>MGSSHHHHHHSQDPGFEFTLMVVGESGLGKSTLINSLFLTDLYSPEYPGPSHRIKKTVQVEQSKVLIKEGGVQLLLTIVDTPGFGDAVDNSNCWQPVIDYIDSKFEDYLNAESRVNRRQMPDNRVQCCLYFIAPSGHGLKPLDIEFMKRLHEKVNIIPLIAKADTLTPEECQQFKKQIMKEIQEHKIKIYEFPETDDEEENKLVKKIK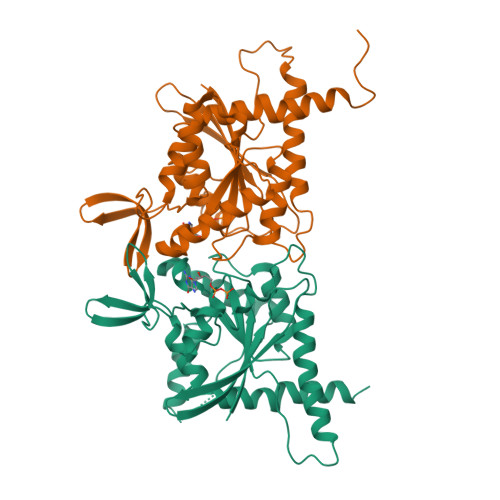DRLPLAVVGSNTIIEVNGKRVRGRQYPWGVAEVENGEHCDFTILRNMLIRTHMQDLKDVTNNVHYENYRSRKLAAVT[2x];>MGFDFNIMVVGQSGLGKSTLVNTLFKSQVSRKASSWNREEKIPKTVEIKAIGHVIEEGGVKMKLTVIDTPGFGDQINNENCWEPIEKYINEQYEKFLKEEVNIARKKRIPDTRVHCCLYFISPTGHSLRPLDLEFMKHLSKVVNIIPVIAKADTMTLEEKSEFKQRVRKELEVNGIEFYPQKEFDEDLEDKTENDKIRQESMPFAVVGSDKEYQVNGKRVLGRKYPWGIIEVENLNHCEFALLRDFVIRTHLQDLKEVTHNIHYETYRAKRLNDNGGLPPVSVDTEESHDSNP[2x]> MVPISPIETVPVKLKPGMDGPKVKQWPLTEEKIKALVEICTEMEKEGKISKIGPENPYNTPVFAIKKKDSTKWRKLVDFRELNKRTQDFWEVQLGIPHPAGLKKKKSVTVLDVGDAYFSVPLDEDFRKYTAFTIPSINNETPGIRYQYNVLPQGWKGSPAIFQSSMTKILEPFKKQNPDIVIYQYMDDLYVGSDLEIGQHRTKIEELRQHLLRWGLTTPDKKHQKEPPFLWMGYELHPDKWTVQPIVLPEKDSWTVNDIQKLVGKLNWASQIYPGIKVRQLSKLLRGTKALTEVIPLTEEAELELAENREILKEPVHGVYYDPSKDLIAEIQKQGQGQWTYQIYQEPFKNLKTGKYARMRGAHTNDVKQLTEAVQKITTESIVIWGKTPKFKLPIQKETWETWWTEYWQATWIPEWEFVNTPPLVKLWYQLEKEPIVGAETFYVDGAANRETKLGKAGYVTNKGRQKVVPLTNTTNQKTELQAIYLALQDSGLEVNIVTNSQYA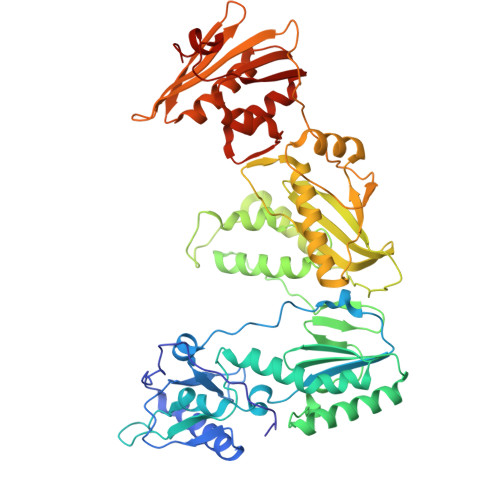LGIIQAQPDKSESELVNQIIEQLIKKEKVYLAWVPAHKGIGGNEQVDKLVSAG> MAKKTSSKGKLPPGPTPLPFIGNYLQLNTEQMYNSLMKISERYGPVFTIHLGPRRVVVLCGHDAVKEALVDQAEEFSGRGEQATFDWLFKGYGVAFSNGERAKQLRRFSIATLRGFGVGKRGIEERIQEEAGFLIDALRGTHGANIDPTFFLSRTVSNVISSIVFGDRFDYEDKEFLSLLRMMLGSFQFTATSTGQLYEMFSSVMKHLPGPQQQAFKELQGLEDFIAKKVEHNQRTLDPNSPRDFIDSFLIRMQEEEKNPNTEFYLKNLVMTTLNLFFAGTETVSTTLRYGFLLLMKHPEVEAKVHEEID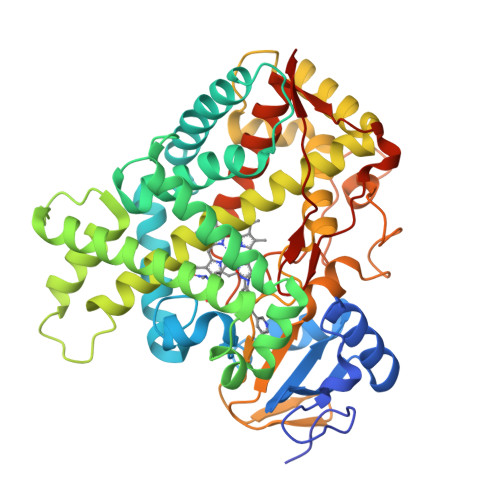RVIGKNRQPKFEDRAKMPYTEAVIHEIQRFGDMLPMGLAHRVNKDTKFRDFFLPKGTEVFPMLGSVLRDPRFFSNPRDFNPQHFLDKKGQFKKSDAFVPFSIGKRYCFGEGLARMELFLFFTTIMQNFRFKSPQSPKDIDVSPKHVGFATIPRNYTMSFLPRHHHH>[2x]MAHHHHHHVDDDDKMVHHDGFQTVKATIDWEHPMFKLYEKAKRNGKWNPADIDFSQDQKDFASLTSEEKISALPLVAGFSAGEEAATLDILPMAHALARQGRLEDVLFLTTFMHDEAKHVEMFSRWQQAVGIGQMDLSVFHNDHYKRIFYEALPEAMNRLYADDSPEAVIRAATVYNMIVEGTLAESGYYTFRQIYKKAGLFPGLLQGIDYLNMDEGRHIQFGIYTIQRIVNED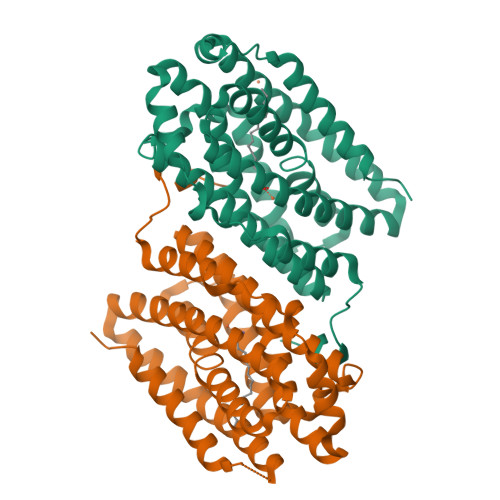ERYYELFIRYMDELWPHVIGYVDYLTELGKRQQQLARTYALEIDYDLLRHYVIKQFNLRKKQISRTKRVDVVEGLEKTAAES>[2x]HHHHHHFNLPPGNYKKPKLLYCSNGGHFLRILPDGTVDGTRDRSDQHIQLQLSAESVGEVYIKSTETGQYLAMDTDGLLYGSQTPNEECLFLERLEENHYN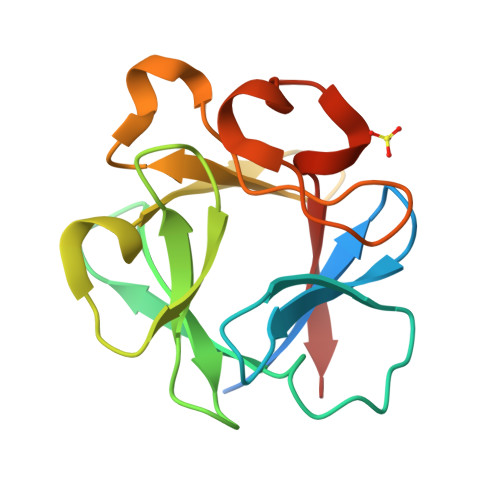TYISKKHAEKGWFVGLKKNGSCKRGPRTHYGQKAILFLPLPVSSD6-[4-[(7-chloranyl-1,2,3,4-tetrahydroacridin-9-yl)amino]butyl]-2-[(oxidanylamino)methyl]pyridin-3-ol 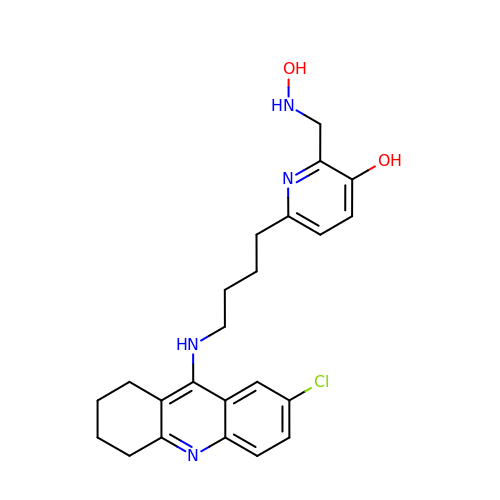| C23 H27 Cl N4 O2 | RLEDPUMYLSBQMO-UHFFFAOYSA-N GH19 chitinase hydrolyzes the glycosidic bonds of chitin, namely beta-1, 4-linked N-acetyl-D-glucosamine. One of the physiological roles of chitinase is to defend plants against pathogenic fungi by degrading chitin, a major component of the cell wall of many fungi. By revealing the evolutionary history and loops appearance of GH19 chitinase, we discover that one loop which is remote from the catalytic site, is necessary to acquire the new antifungal activity. We demonstrate that this remote loop directly accesses the fungal cell wall, and surprisingly, it needs to adopt a defined structure supported by long-range intramolecular interactions to perform its function.

To investigate the contribution to the antifungal activity of the 45 substitutions, we constructed mutants of Anc4 + Loop II with substitutions in proximity to loop II. We chose six substitutions within 4.0 Å from Loop II and introduced them accordingly to their proximity to each other’s (Fig. 4C, D: mutations A, p12K and n13H; mutation B, s58T mutations C, n193G, y194F, and d197R). C The crystal structure of Anc4 + Loop II integrated with all six substitutions (p12K, n13H, s58T, n193G, y194F, and d197R) revealed the interactions of these residues with loop II. Mutations A, B, and C increased antifungal activity 4.7, 1.2, and 5.4-fold, respectively. These substitutions increased antifungal activity while retaining the same degree of chitinase activity. Cell wall binding activity assay confirmed that integrating these mutations increased binding activity to the fungal cell wall. MD simulations of these mutants revealed a gradual reduction of loop II flexibility directly related to the introduction of these six substitutions Furthermore, these substitutions decreased only the mobility of loop II not the one of a loop region between the ninth and tenth α-helices (positions 192–201). Furthermore, crystal structures of Anc4 + Loop II + A and Anc4 + Loop II + A + B + C revealed that their loop II structures are retained as in the structure of Anc5’s loop II, namely the antifungal active variant. Altogether, these results exemplify that antifungal activity enhanced by cell wall binding activity is supported by the substitutions that rigidify loop II. Our mutational analysis revealed that some of substitutions are conserved in loopful-type GH19 chitinases and six substitutions are needed to perform new function.

> MVSRSMFDQLFKHRNSFYTYDAFIAAAKSFPSFGTTGDTDVRKREIAAFFAHVSHETTGGWPTAPDGPYAWGLVYIEEINQSNDYCDPSTQYPCAPGKQYYGRGPLQLSWNYNYGPCGDALGLDLLNNPDLVAQDPVIAFKTALWFWMTPQSPKPSCHDVMTGNWTPSSADLAAGRVPGFGVTTNIINGGLECGKGNPAQAENRVGFYKRFCNQLGVSPGSNLDCANMRPFG The ability of bacteria to maintain appreciable amounts of intracellular copper has only recently been discovered. This is achieved by a family of copper storage proteins (the Csps), which are tetramers of four‐helix bundles possessing Cys‐lined cavities binding up to approximately 20 CuI ions per monomer. The twin‐arginine translocated Csps (MtCsp1 and MtCsp2) from the methanotroph Methylosinus trichosporium OB3b are involved in copper storage for the main methane‐oxidizing enzyme. This organism also possesses a Csp3 (MtCsp3), homologues of which are much more widespread and allow bacteria to accumulate cytosolic copper. MtCsp1 has 13 Cys residues and binds a similar number of CuI ions, whereas MtCsp3 has 18 Cys residues and accommodates 19 CuI ions. Thiolate‐coordinated CuI clusters are remarkably rare in biological systems, but the crystallization of MtCsp3 in the presence of increasing amounts of CuI provides unprecedented insight into how such species form in a protein and are used to drive copper storage.

The crystal structure of MtCsp3 plus ca. 2 molar equiv of CuI (see Supporting Information6, 7, 13, 14, 15) has four partially occupied sites. These are Cu11 with an occupancy of 0.25, and Cu12, Cu13, and Cu14, all with occupancies of 0.35, which form a symmetrical tetranuclear cluster. Cu12 and Cu14 are bound by the Cys residues of CXXXC motifs, that is, from the same α‐helix, whilst Cu11 and Cu13 are ligated by Cys residues on different helices (Cu13 is also weakly coordinated by Asn 58). The thiolates of Cys 97, Cys 101, Cys 114, and Cys 118 bridge between two CuI ions (μ2‐S‐Cys). Additional stabilization is provided by CuI–CuI interactions (ca. 2.6–2.7 Å) between neighboring metal ions. There is no preference for CuI binding at a particular tetranuclear cluster apart from in the structure plus ca. 2 equiv, in which only Cu11–Cu14 is occupied. This must be due to the fact that as CuI ions diffuse past Cu15 to Cu19 at the mouth of the bundle, Cu11–Cu14 are the first sites they encounter at which they can form a tetranuclear cluster. The position of Cu11 in 2 equiv MtCsp3 corresponds to Cu11b in the 8  and 14 equiv structures, which is therefore bound before Cu11a. We identify [Cu4(μ2‐S‐Cys)4] as an intermediate for the three clusters that are made up of the first sites (Cu3 to Cu14) to be occupied in MtCsp3.

> MHVEAMISKHPQARGQTDRSLVQCVEMCFDCAQTCAACADACLGEDKVADLRHCIRLNLDCAEICVAAGSIASRAAGTEESILRTMLQTCAEMCRMCEEECRRHAGNHEHCRICADVCKECETACRSATGLTH> GGGGUGUGCCCGGCAUGGGUGCAGUCUAUAGGGUGAGAGUCCCGAACUGUGAAGGCAGAAGUAACAGUUAGCCUAACGCAAGGGUGUCCGUGGCGACAUGGAAUCUGAAGGAAGCGGACGGCAAACCUUCGGUCUGAGGAACACGAACUUCAUAUGAGGCUAGGUAUCAAUGGAUGAGUUUGCAUAACAAAACAAAGUCCUUUCUGCCAAAGUUGGUACAGAGUAAAUGAAGCAGAUUGAUGAAGGGAAAGACUGCAUUCUUACCCGGG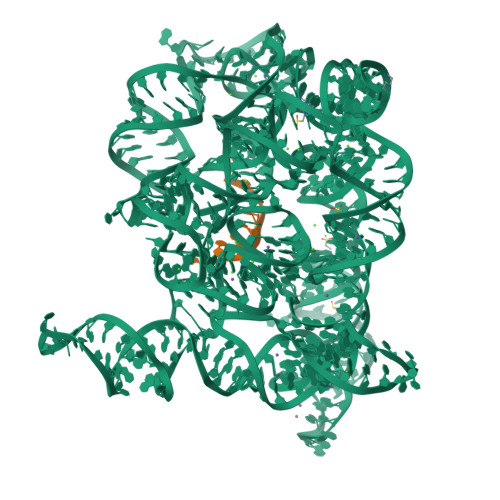GAGGUCUGGAAACAGAAGUCAGCAGAAGUCAUAGUACCCUGUUCGCAGGGGAAGGACGGAACAAGUAUGGCGUUCGCGCCUAAGCUUGAACCGCCGUAUACCGAACGGUACGUACGGUGGUGUG;> AUUUAUUA> GSHMRNELEEMQRRADQLADESLESTRRMLQLVEESKDAGIRT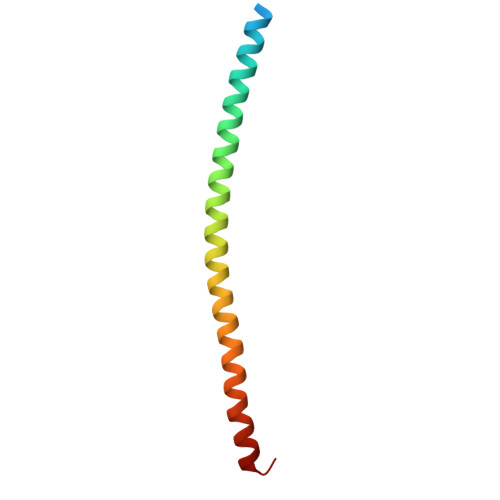LVMLDEQGEQLDRVEEGMNHINQDMKEAEKNLKDLGK>[3x]MDLKILSLATDKTTDKLQEFLQTLKDDDLASLLQNQAVKGRAVGTLLRAVLKGSPCSEEDGALRRYKIYSCCIQLVESGDLQQDVASEIIGLLMLEVHHFPGPLLVDLASDFVGAVREDRLVNGKSLELLPIILTALATKKEVLACGKGDLNGEEYKRQLIDTLCSVRWPQRYMIQLTSVFKDVCLTPEEMNLVVAKVLTMFSKLNLQEIPPLVYQLLVLSSKGSRRSVLDGIIAFFRELDKQHREEQSSDELSELITAPADELYHVEGTVILHIVFAIKLDCELGRELLKHLKAGQQGDPSKCLCPFSIALLLSLTRIQRFEEQVFDLLKTSVVKSFKDLQLLQGSKFLQTLVPQRTCVSTMILEVVRNSVHSWDHVTQGLIEFGFILMDSYGPKKILDGKAVEIGTSLSKMTNQHACKLGANILLETFKIHEMIRQEILEQVLN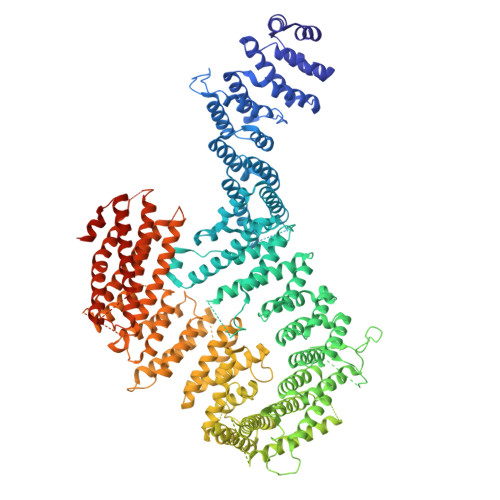RVVTRTSSPINHFLDLFSDIIMYAPLILQNCSKVTETFDYLTFLPLQTVQGLLKAVQPLLKISMSMRDSLILVLRKAMFASQLDARKSAVAGFLLLLKNFKVLGSLPSSQCTQSIGVTQVRVDVHSRYSAVANETFCLEIIDSLKRSLGQQADIRLMLYDGFYDVLRRNSQLASSIMQTLFSQLKQFYEPEPDLLPPLKLGACVLTQGSQIFLQEPLDHLLSCIQHCLAWYKSRVVPLQQGDEGEEEEEELYSELDDMLESITVRMIKSELEDFELDKSADFSQNTNVGIKNNICACLIMGVCEVLMEYNFSISNFSKSKFEEILSLFTCYKKFSDILSEKAGKGKAKMTSKVSDSLLSLKFVSDLLTALFRDSIQSHEESLSVLRSSGEFMHYAVNVTLQKIQQLIRTGHVSGPDGQNPDKIFQNLCDITRVLLWRYTSIPTSVEESGKKEKGKSISLLCLEGLQKTFSVVLQFYQPKVQQFLQALDVMGTEEEEAGVTVTQRASFQIRQFQRSLLNLLSSEEDDFNSKEALLLIAVLSTLSRLLEPTSPQFVQMLSWTSKICKEYSQEDASFCKSLMNLFFSLHVLYKSPVTLLRDLSQDIHGQLGDIDQDVEIEKTDHFAVVNLRTAAPTVCLLVLSQAEKVLEEVDWLIAKIKGSANQETLSDKVTPEDASSQAVPPTLLIEKAIVMQLGTLVTFFHELVQTALPSGSCVDTLLKGLSKIYSTLTAFVKYYLQVCQSSRGIPNTVEKLVKLSGSHLTPVCYSFISYVQNKSSDAPKCSEKEKAAVSTTMAKVLRETKPIPNLVFAIEQYEKFLIQLSKKSKVNLMQHMKLSTSRDFKIKGSVLDMVLREDEEHHHHHH>MELIRIAMKKDLENDNSLMNKWATVAGLKNPNPLYDFLNHDGKTFNEFSSIVNIVKSQYPDREYELMKDYCLNLDVKTKAARSALEYADANMFFEIEDVLIDSMISCSNMKSKEYGKVYKIHRELSNSVITEFEAVKRLGKLNIKTPEMNSFSRLLLLYHYLSTGNFSPMAQLIKQIDLSEISENMYIRNTYQTRVHVLMSNIKLNENSLEECREYSKKALESTNILRFQVFSYLTIGNSLLFSNYELAQENFLKGLSISVQNENYNMIFQQALCFLNNVWRKENKWINFESDSIMDLQEQAHCFINFNENSKAKEVLDKLDLLVHNDNELAMHYYLKGRLEQNKACFYSSIEYFKKSNDKFLIRLPLLELQKMGENQKLLELLLL[2x]

Bacillus phages use a communication system, termed “arbitrium,” to coordinate lysis-lysogeny decisions. Arbitrium communication is mediated by the production and secretion of a hexapeptide (AimP) during lytic cycle. Once internalized, AimP reduces the expression of the negative regulator of lysogeny, AimX, by binding to the transcription factor, AimR, promoting lysogeny. We have elucidated the crystal structures of AimR from the Bacillus subtilis SPbeta phage in its apo form, bound to its DNA operator and in complex with AimP.

To understand how AimR binds to its unusual operator sequence, we determined the crystal structure of SPbeta AimR bound to a 43-bp DNA fragment, including the AimR operator characterized here. SPbeta AimR-DNA crystals belong to space group I4122 and diffracted to 2.2 Å resolution. The asymmetric unit contains two AimR molecules arranged as a dimer and an operator-DNA molecule. However, the relative disposition between the TPRN-ter and TPRC-ter subdomains is slightly different from that observed in the apo form, and this is reflected in rmsd differences when monomers from these structures are compared (rmsd from 0.92 to 2.06 Å), confirming the AimR plasticity. As a result of this flexibility, the HTH domain’s disposition changes and the DNA recognition helices α3 increase its separation (1–8 Å) with respect to the apo structures. Similar to other HTH-type DNA binding proteins, the recognition helix α3 from the HTH motif inserts into the DNA major groove. Direct readout of the DNA is accomplished via the side chains of residues N30, N32, and Y35, which interact mainly with the T5C6A7/A35G36T37 motif of the SPbeta AimR box. The K79 and R82 from helix α6 in TPR1 as well as N109, N143, and K145 placed in the loops connecting the helices of TPR2 and TPR3 interact with the DNA backbone. These nonspecific interactions are distributed along the two DNA turns generated by the 25-bp spacer and help to maintain an extended conformation and induce some distortion in the DNA. The AimR binding also induces a small bend (around 20°) over the entire operator, with the concave side of the DNA facing the protein and the double G/C pair in the convex kink.> RRPVTVLGLGAMGRALAGALVAAGHPTTVWNRTPGRAAALTAAGATEAGTAAEAVAAGDLVVVCLLDDEVTRQVLALVAPVLAGRTLVNLTNGTPEQARRLAEWATSHGADHLDGGIMAVPAMIGQPGALILYSGPEDVFRAGRETLAAFGAAHWLGADPGAAALHDLALLAAMYGMFGGYLHAVAMIRAAGVPATGFTPLATDWLTAMLGALPALARGVDSGDH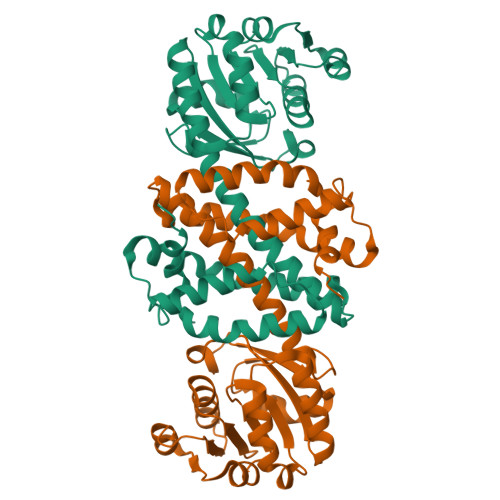AADGSAVGMQAAAFGNLLAASREGGVSTSLLEPVRRLLDDAVRAGHGADGLSALVDLLRQS>[4x]AVSKVYARSVYDSRGNPTVEVELTTEKGVFRSIVPSGANTGVHEALEMRDGDKSKWMGKGVLHAVKNVNDVIAPAFVKANIDVKDQKAVDDFLISLDGTANKSKLGANAILGVSLAASRAAAAEKNVPLYKHLADLSKSKTSPYVLPVPFLNVLNGGSHAGGALALKEFMIAPTGAKTFAEALRIGSEVYHNLKSLTKKRYGASAGNVGDEGGVAPNIQTAEEALDLIVDAIKAAGHDGKIK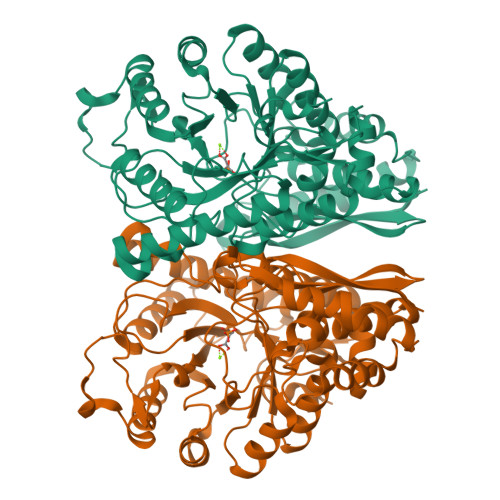IGLDCASSEFFKDGKYDLDFKNPNSDKSKWLTGPQLADLYHSLMKRYPIVSIEDPFAEDDWEAWSHFFKTAGIQIVADRLTVTNPKRIATAIEKKAADALLLKVNQIGTLSESIKAAQDSFAAGWGVMVSHRSGETEDTFIADLVVGLRTGQIKTGAPARSERLAKLNQLLRIEEELGDNAVFAGENFHHGDKLLHHHHHH> VVRVADTMPSGPSNSESIPALTAAETGHTSQVVPSDTIQTRHVRNFHVRSESSVENFLSRSACVYIVEYKTRDDTPDKMYDSWVINTRQVAQLRRKLEFFTYVRFDVEVTFVITSVQDDSTRQNTDTPALTHQIMYVPPGGPIPQAVDDYNWQTSTNPSVFWTEGNAPPRMSIPFMSVGNAYSNFYDGWSHFSQTGVYGFNTLNNMGKLYFRHVNDKTI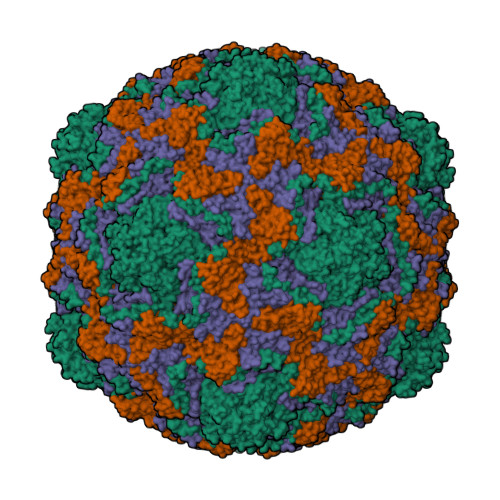SPITSKVRIYFKPKHVKAWVPRPPRLCEYTHKDNVDFEPKGVTTSRTQLTISNSTH;> SDRVRSITLGNSTITTQESANVVVGYGVWPDYLSDEEATAEDQPTQPDVATCRFYTLDSVSWMKESQGWWWKFPDALRDMGLFGQNMQYHYLGRSGYTIHVQCNASKFHQGCLLVVCVPEAEMGAANINEKINREHLSNGEVANTFSGTKSSNTNDVQQAVFNAGMGVAVGNLTIFPHQWINLRTNNCATIVMPYINSVPMDNMFRHYNFTLMIIPFAKLDYAAGSSTYIPITVTVAPMCAEYNGLRLAGHQ;> GLPVMNTPGSNQFLTSDDYQSPTAMPQFDVTPEMNIPGEVKNLMEIAEVDSVVPVNNVNENVNSLEAYRIPVHSVTETGAQVFGFTLQPGADTVMERTLLGEILNYYANWSGSIKLTFMYCGSAMATGKFLLAYSPPGAGVPKNRREAMLGTHIIWDIGLQSSCVLCVPWISQTHYRFVSKDIYTDAGFITCWYQTSIVVPAEVQNQSVILCFVSACNDFSVRLLRDSPFVRQTAFYQ;> GAQVSTQKTGAHETSLSASGNSTIHYTNINYYKDAASNSANRQDFTQDPGKFTEPVKDIMVKSLPALN>[2x]HFLCGVVEGFYGRPWVMEQRKELFRRLQKWELNTYLYAPKDDYKHRMFWREMYSVEEAE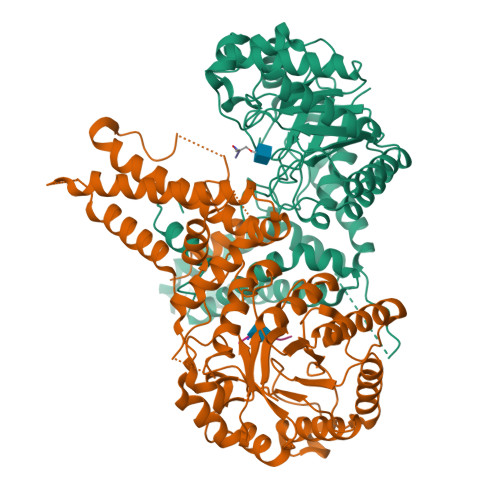QLMTLISAAREYEIEFIYAISPGLDITFSNPKEVSTLKRKLDQVSQFGCRSFALLFDNIDHNMCAADKEVFSSFAHAQVSITNEIYQYLGEPETFLFCPTEYCGTFCYPNVSQSPYLRTVGEKLLPGIEVLWTGPKVVSKEIPVESIEEVSKIIKRAPVIWDNIHANDYDQKRLFLGPYKGRSTELIPRLKGVLTNPNCEFEANYVAIHTLATWYKSNMNGVRKDVVMTDSEDSTVSIQIKLENEGSDEDIETDVLYSPQMALKLALTEWLQEFGVPHQYSSRGGGGSGGGGSVTLEDLQLLADLFYLPYEHGPKGAQMLREFQWLRANSSVVSVNCKGKDSEKIEEWRSRAAKFEEMCGLVMGMFTRLSNCANRTILYDMYSYVWDIKSIMSMVKSFVQWLGCRSHSSAQFLIGDQEPWAFRGGLAGEFQRLLPIDGANDLFFQ;>FPTSTSLSPFYLR[2x]>YFQSMGALIPEPEVKIEVLQKPFICHRKTKGGDLMLVHYEGYLEKDGSLFHSTHKHNNGQPIWFTLGILEALKGWDQGLKGMCVGEKRKL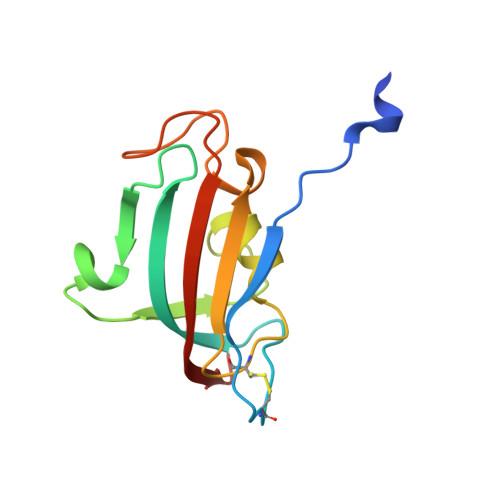IIPPALGYGKEGKGKIPPESTLIFNIDLLEIRNGP[10x]> ALADRFAELERRYDARLGVYVPATGTTAAIEYRADERFAFCSTFKAPLVAAVLHQNPLTHLDKLITYTSDDIRSISPVAQQHVATGMTIGQLCDAAIRYSDGTAANLLLADLGGPGGGTAAFTGYLRSLGDTVSRLDAEEPELARDPPGDERDTTTPHAIALV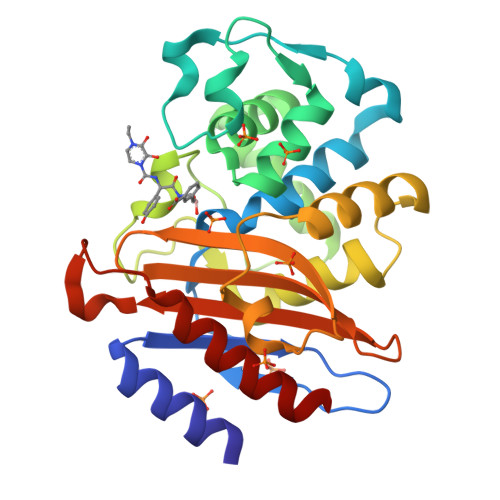LQQLVLGNALPPDKRALLTDWMARNTTGAKRIRAGFPADWKVIDKTGTGDYGRANDIAVVWSPTGVPYVVAVMSDRAGGGYDAEPREALLAEAATCVAGVLA>[2x]MELHHHHHHEEMPFKPLVTAGIESLLNTFLYRSPALKTARSRLLGKVLRVEVKGFSTSLILVFSERQV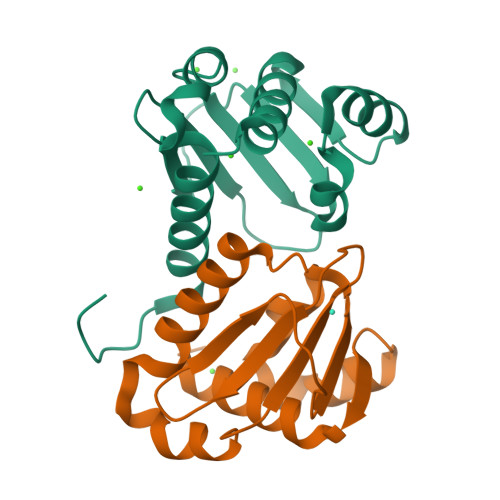DVLGEWAGDADCTVIAYASVLPKLRDRQQLTALIRSGELEVQGDIQVVQNFVALADLAEFDPA> PEGERKNNNKRWYFTREQLENSPSRRFGVDPDKELSYRQQAANLLQDMGQRLNVSQLTINTAIVYMHRFYMIQSFTRFPGNSVAPAALFLAAKVEGQPKKLEHVIKVAHTCLHPQESLPDTRSEAYLQQVQDLV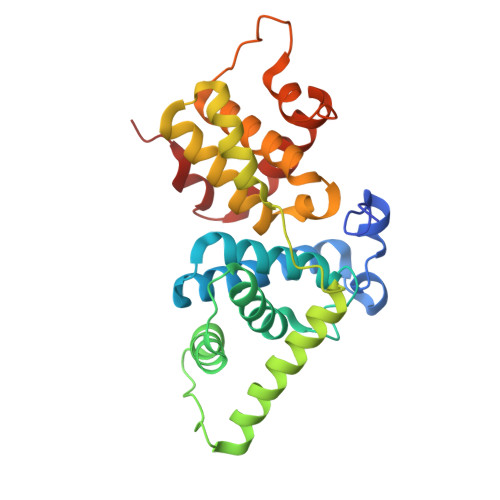ILESIILQTLGFELTIDHPHTHVVKCTQLVRASKDLAQTSYFMATNSLHLTTFSLQYTPPVVACVCIHLACKWSNWEIPVSTDGKHWWEYVDATVTLELLDELTHELLQILEKTPNRLKRIWNWR>GPHMPEFKVDARGPIEIWTIDGESRRNAISRAMLKELGELVTRVSSSRDVRAVVITGAGDKAFCAGADLKERATMAEDEVRAFLDGLRRTFRAIEKSDCVFIAAINGAALGGGTELALACDLRVAAPAAELGLTEVKLGIIPGGGGTQRLARLVGPGRAKDLILTARRINAAEAFSVGLANRLAPEGHLLAVAYGLAESVVENAPIAVATAKHAIDEGTGLELDDALA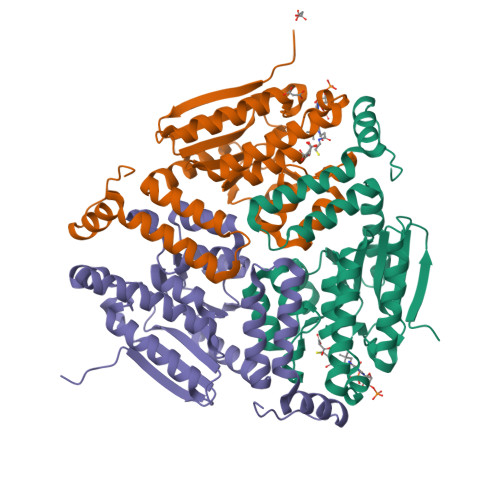LELRKYEEILKTEDRLEGLRAFAEKRAPVYKGR[3x]>MSSFLHIGDIVSLYAEGSVNGFISTLGLVDDRCVVEPAAGDLDNPPKKFRDCLFKVCPMNRYSAQKQYWKAKQTKQDKEKIADVVLLQKLQHAAQMEQKQNDTENKKVHGDVVKYGSVIQLLHMKSNKYLTVNKRLPALLEKNAMRVTLDATGNEGSWLFIQPFWKLRSNGDNVVVGDKVILNPVNAGQPLHASNYELSDNAGCKEVNSVNCNTSWKINLFMQFRDHLEEVLKGGDVVRLFHAEQEKFLTCDEYKGKLQVFLRTTLRQSATSATSSNALWEVEVVHHDPCRGGAGHWNGLYRFKHLATGNYLAAEENPSYKGDASDPKAAGMGAQGRTGRRNAGEKIKYCLVAVPHGNDIASLFELDPTTLQKTDSFVPRNSYVRLRHLCTNTWIQSTNVPIDIEEERPIRLMLGTCPTKEDKEAFAIVSVPVSEIRDLDFANDASSMLASAVEKLNEGFISQNDRRFVIQLLEDLVFFVSDVPNNGQNVLDIMVTKPNRERQKLMREQNILKQVFGILKAPFREKGGEGPLVRLEELSDQKNAPYQHMFRLCYRVLRHSQEDYRKNQEHIAKQFGMMQSQIGYDILAEDTITALLHNNRKLLEKHITKTEVETFVSLVRKNREPRFLDYLSDLCVSNHIAIPVTQELICKCVLDPKNSDILIRTELRPVKEMAQSHEYLSIEYSEEEVWLTWTDKNNEHHEKSVRQLAQEARAGNAHDENVLSYYRYQLKLFARMCLDRQYLAIDEISQQLGVDLIFLCMADEMLPFDLRASFCHLMLHVHVDRDPQELVTPVKFARLWTEIPTAITIKDYDSNLNASRDDKKNKFANTMEFVEDYLNNVVSEAVPFANEEKNKLTFEVVSLAHNLIYFGFYSFSELLRLTRTLLGIIDCVQGPPAMLQAYEDPGGKNVRRSIQGVGHMMSTMVLSRKQSVFSAPSLSAGASAAEPLDRSKFEENEDIVV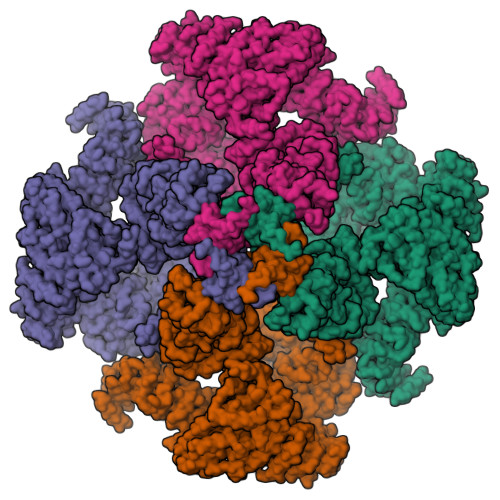METKLKILEILQFILNVRLDYRISYLLSVFKKEFVEVFPMQDSGADGTAPAFDSTTANMNLDRIGEQAEAMFGVGKTSSMLEVDDEGGRMFLRVLIHLTMHDYAPLVSGALQLLFKHFSQRQEAMHTFKQVQLLISAQDVENYKVIKSELDRLRTMVEKSELWVDKKGSGKGEEVEAGAAKDKKERPTDEEGFLHPPGEKSSENYQIVKGILERLNKMCGVGEQMRKKQQRLLKNMDAHKVMLDLLQIPYDKGDAKMMEILRYTHQFLQKFCAGNPGNQALLHKHLHLFLTPGLLEAETMQHIFLNNYQLCSEISEPVLQHFVHLLATHGRHVQYLDFLHTVIKAEGKYVKKCQDMIMTELTNAGDDVVVFYNDKASLAHLLDMMKAARDGVEDHSPLMYHISLVDLLAACAEGKNVYTEIKCTSLLPLEDVVSVVTHEDCITEVKMAYVNFVNHCXXXXXXXXXXXXXXXXDYKNIIEKLQDIITALEERLKPLVQAELSVLVDVLHWPELLFLEGSEAYQRCESGGFLSKLIQHTKDLMESEEKLCIKVLRTLQQMLLKKTKYGDRGNQLRKMLLQNYLQNRKSTSRGDLPDPIGTGLDPDWSAIAATQCRLDKEGATKLVCDLITSTKNEKIFQESIGLAIHLLDGGNTEIQKSFHNLMMSDKKSERFFKVLHDRMKRAQQETKSTVAVNMNDLGSQPHEDREPVDPTTKGRVASFSIPGSSSRYSLGPSLRRGHEVSERVQSSEMGTSVLIMQPILRFLQLLCENHNRDLQNFLRCQNNKTNYNLVCETLQFLDIMCGSTTGGLGLLGLYINEDNVGLVIQTLETLTEYCQGPCHENQTCIVTHESNGIDIITALILNDISPLCKYRMDLVLQLKDNASKLLLALMESRHDSENAERILISLRPQELVDVIKKAYLQEEERENSEVSPREVGHNIYILALQLSRHNKQLQHLLKPVKRIQEEEAEGISSMLSLNNKQLSQMLKSSAPAQEEEEDPLAYYENHTSQIEIVRQDRSMEQIVFPVPGICQFLTEETKHRLFTTTEQDEQGSKVSDFFDQSSFLHNEMEWQRKLRSMPLIYWFSRRMTLWGSISFNLAVFINIIIAFFYPYMEXXXXXXXXXPLIVALILRSIYYLGIGPTLNILGALNLTNKIVFVVSFVGNRGTFIRGYKAMVMDMEFLYHVGYILTSVLGLFAHELFYSILLFDLIYREETLFNVIKSVTRNGRSILLTALLALILVYLFSIVGFLFLKDDFILEVDRLPNNHSTASPLGMPHGAAAFVDTCSGDKMDCVSGLSVPEVLEEDRELDSTERACDTLLMCIVTVMNHGLRNGGGVGDILRKPSKDESLFPARVVYDLLFFFIVIIIVLNLIFGVIIDTFADLRSEKQKKEEILKTTCFICGLERDKFDNKTVSFEEHIKLEHNMWNYLYFIVLVRVKNKTDYTGPESYVAQMIKNKNLDWFPRMRAMSLVXXXXXXXXXXXXXXXXXXXXX[4x]> MAYTTFSQTKNDQLKEPMFFGQPVNVARYDQQKYDIFEKLIEKQLSFFWRPEEVDVSRDRIDYQALPEHEKHIFISNLKYQTLLDSIQGRSPNVALLPLISIPELETWVETWAFSETIHSRSYTHIIRNIVNDPSVVFDDIVTNEQIQKRAEGISSYYDELIEMTSYWHLLGEGTHTVNGKTVTVSLRELKKKLYLCLMSVNALEAIRFYVSFACSFAFAERELMEGNAKIIRLIARDEALHLTGTQHMLNLLRSGADDPEMAEIAEECKQECYDLFVQAAQQEKDWADYLFRDGSMIGLNKDILCQYVEYITNIRMQAVGLDLPFQTRSNPIPWINTWLVSDNVQVAPQEVEVSSYLVGQIDSEVDTDDLSNFQL

Here, we present a novel polymer-based support and an associated deposition method, with the aim of providing ultralow-background conditions for serial data collection. The supports themselves consist of a thin 2–3 µm thick cyclic olefin co­polymer (COC) membrane perforated with a dense array of 2–3 µm sized holes and suspended on a rigid frame. To assess the quality of structures that can be obtained from chip-mounted crystals, diffraction data were collected from a range of proteins. These proteins included the insulin, thaumatin and HEWL that were used in initial tests, and also TD1, a tubulin–DARPin D1 complex, EcR2a, a class Ia ribo­nucleotide reductase radical-generating subunit, rhodopsin–miniGo and PepTst, a bacterial peptide transporter.

TD1 and EcR2a are both soluble proteins with crystals grown using vapor diffusion, rhodopsin–miniGo is a membrane protein with crystals grown in vapor-diffusion plates and PepTst is a membrane protein where crystals are obtained using LCP methods. In some cases, such as EcR2a and the membrane-protein complex rhodopsin–miniGo, direct deposition provided satisfactory results. The data collected from proteins loaded onto the chips compares favorably with similar structures in the Protein Data Bank (PDB). It was interesting to contrast the data collected by small rotations with the stills data. Although a detailed comparison between these two data-collection modes was limited by the different data-processing software, doses per position (ten times higher for the wedges) etc., the final resolutions were similar. This suggests that the intrinsic diffraction limit of the samples using this preparation method may have been reached with both data-collection methods.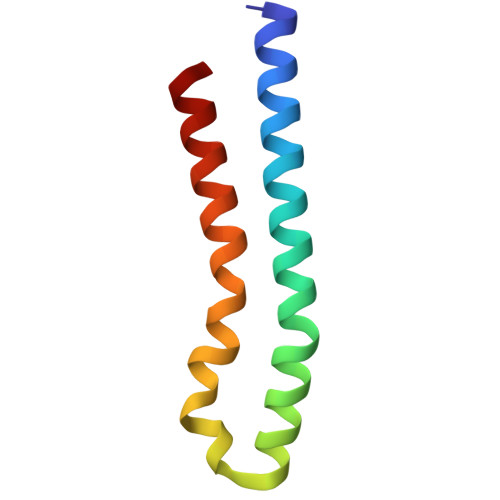> GGLDRGLIAVGMGLAVGLAALGTGVAQARIGAAGVGAIAEDRSNFGTALIFLLLPETLVIFGLLIAFILNGRL> MSTDTSGVGVREIDAGALPTRYARGWHCLGVAKDYLEGKPHGVEAFGTKLVVFADSHGDLKVLDGYCRHMGGDLSEGTVKGDEVACPFHDWRWGGDGRCKLVPYARRTPRMARTRSWTTDVRSGLLFVWHDHEGNPPDPAVRIPEIPEAASDEWTDWRWNRILIEGSNCRDIIDNVTDMAHFFYIHFG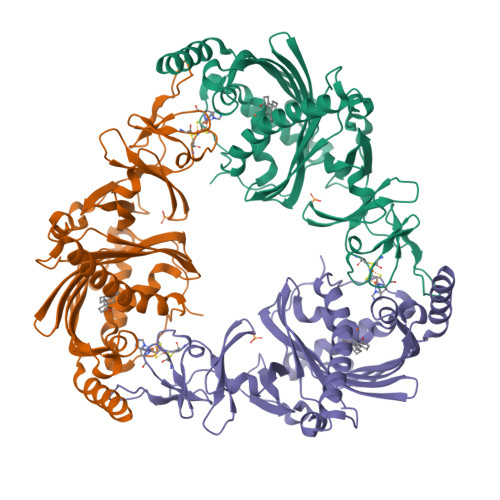LPTYFKNVFEGHIASQYLHNVGRPDVDDLGTSYGEAHLDSEASYFGPSFMINWLHNRYGNYKSESILINCHYPVTQNSFVLQWGVIVEKPKGMSEEMTDKLSRVFTEGVSKGFLQDVEIWKHKTRIDNPLLVEEDGAVYQLRRWYEQFYVDVADIKPEMVERFEIEVDTKRANEFWNAEVEKNLKSREVSDDVPAEQH>TIPSEIINWTILNEIISMDDDDSDFSKGLIIQFIDQAQTTFAQMQRQLDGEKNLTELDNLGHFLKGSSAALGLQRIAWVCERIQNLGRKMEHFFPNKTELVNTLSDKSIINGINI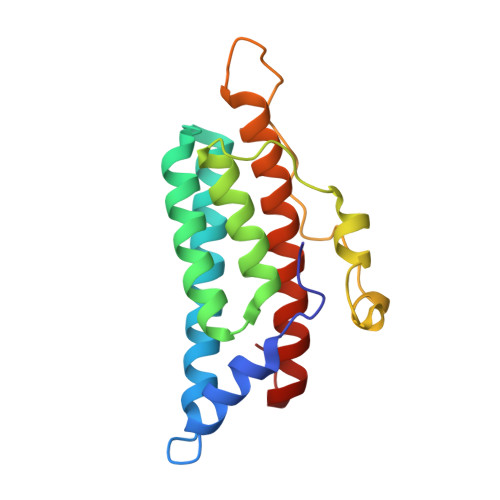DEDDEEIKIQVDDKDENSIYLILIAKALNQSRLEFKLARIELSKYYNTNL[2x]>HMGARASVLSGGELDKWEKIRLRPGGKKQYKLKHIVWASRELERFAVNPGLLETSEGCRQILGQLQPSLQTGSEELRSLYNTI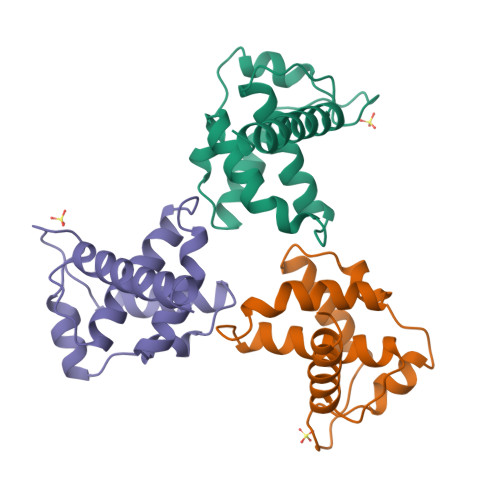AVLYCVHQRIDVKDTKEALDKIEEEQNKSKKKAQQAAADTGNNSQVSQNY[6x]>MKEFYISIETVGNNIVERYIDENGKERTREVEYLPTMFRHCKEESKYKDIYGKNCAPQKFPSMKDARDWMKRMEDIGLEALGMNDFKLAYISDTYGSEIVYDRKFVRVANCDIEVTGDKFPDPMKAEYEIDAITHYDSIDDRFYVFDLLNSMYGSVSKWDAKLAAKLDCEGGDEVPQEILDRVIYMPFDNERDMLMEYINLWEQKRPAIFTGWNIEGFAVPYIMNRVKMILGERSMKRFSPIGRVKSKLIQNMYGSKEIYSIDGVSILDYLDLYKKFAFTNLPSFSLESVAQ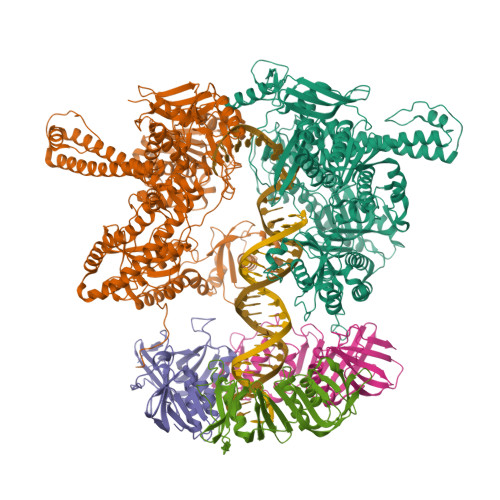HETKKGKLPYDGPINKLRETNHQRYISYNIIDVESVQAIDKIRGFIDLVLSMSYYAKMPFSGVMSPIKTWDAIIFNSLKGEHKVIPQQGSHVKQSFPGAFVFEPKPIARRYIMSFDLTSLYPSIIRQVNISPETIRGQFKVHPIHEYIAGTAPKPSDEYSCSPNGWMYDKHQEGIIPKEIAKVFFQRKDWKKKMFAEEMNAEAIKKIIMKGAGSCSTKPEVERYVKFSDDFLNELSNYTESVLNSLIEECEKAATLANTNQLNRKILINSLYGALGNIHFRYYDLRNATAITIFGQVGIQWIARKINEYLNKVCGTNDEDFIAAGDTDSVYVCVDKVIEKVGLDRFKEQNDLVEFMNQFGKKKMEPMIDVAYRELCDYMNNREHLMHMDREAISCPPLGSKGVGGFWKAKKRYALNVYDMEDKRFAEPHLKIMGMETQQSSTPKAVQEALEESIRRILQEGEESVQEYYKNFEKEYRQLDYKVIAEVKTANDIAKYDDKGWPGFKCPFHIRGVLTYRRAVSGLGVAPILDGNKVMVLPLREGNPFGDKCIAWPSGTELPKEIRSDVLSWIDHSTLFQKSFVKPLAGMCESAGMDYEEKASLDFLFG[2x];>MKLSKDTTALLKNFATINSGIMLKSGQFIMTRAVNGTTYAEANISDVIDFDVAIYDLNGFLGILSLVNDDAEISQSEDGNIKIADARSTIFWPAADPSTVVAPNKPIPFPVASAVTEIKAEDLQQLLRVSRGLQIDTIAITVKEGKIVINGFNKVEDSALTRVKYSLTLGDYDGENTFNFIINMANMKMQPGNYKLLLWAKGKQGAAKFEGEHANYVVALEADSTHDF[3x]> MVECSGNLFTQRTGTITSPDYPNPYPKSSECSYTIDLEEGFMVTLQFEDIFDIEDH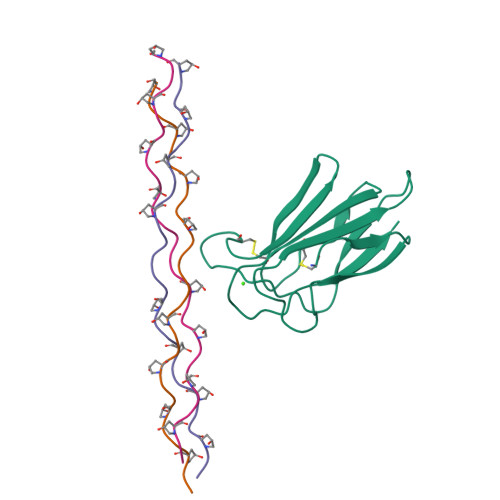PEVPCPYDYIKIKAGSKVWGPFCGEKSPEPISTQSHSIQILFRSDNSGENRGWRLSYRA;>[3x]XGPPGPPGPPGPPGKLGPPGPPGPPGPPX>[4x]GGSVEEIRLPRAGGPLGLSIVGGSDHSSHPFGVQEPGVFISKVLPRGLAA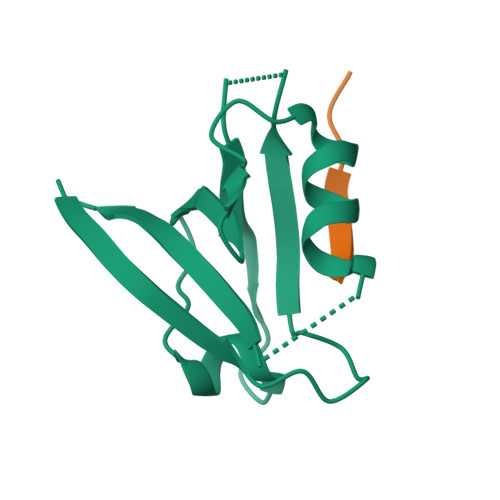RSGLRVGDRILAVNGQDVRDATHQEAVSALLRPCLELSLLVRRD;>[4x]KMARTIESKV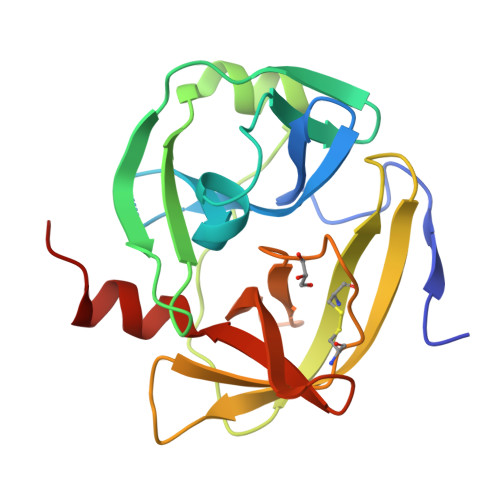> VLGSFYSPVKAGDEPASLVAIKSGPTTIGFGCRTKIDGEDCLLTAHHVWCNSMRPTGLAKAGKQVSVEDWEISMSSSDKMLDFAIVRVPTHVWSKLGVKSTPLVCPSSKDVITCYGGSSSDCLMSGVGSSSTSEFTWKLTHTCPTAAGWSGTPLYSSRGVVGMHVGFEEIGKLNRGVNMFYVANYLLRSNE>[2x]MSKPKQPPDASPANLLTSLVRAHLDSGPSTAKLDYSKFQELVLPHFGKEDAGDVQQFYDLLSGSLEVIRKWAEKIPGFAELSPADQDLLLESAFLELFILRLAYRSKPGEGKLIFCSGLVLHRLQCARGFGDWIDSILAFSRSLHSLLVDVPAFACLSALVLITDRHGLQEPRRVEELQNRIASCLKEHVAAVAGEPQPASCLSRLLGKLPELRTLCTQGLQRIFYLKLEDLVPPPPIIDKIFM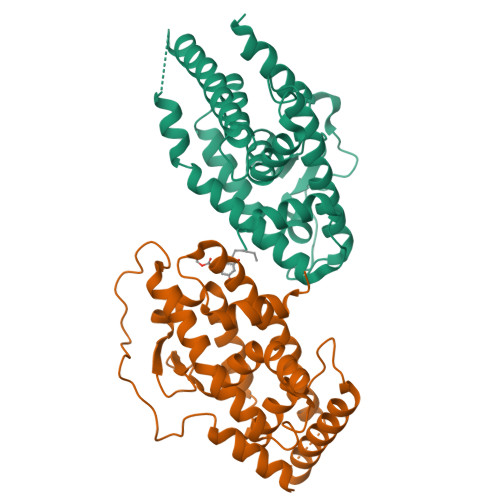DTLPFLEHHHHHH> 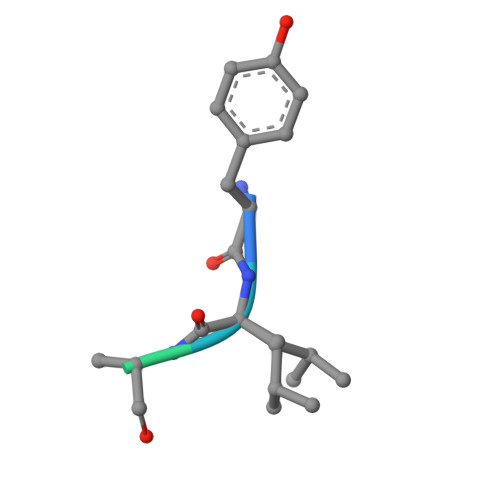YLFVQRDSKE>[2x]SMEDPDQLYTTLKNL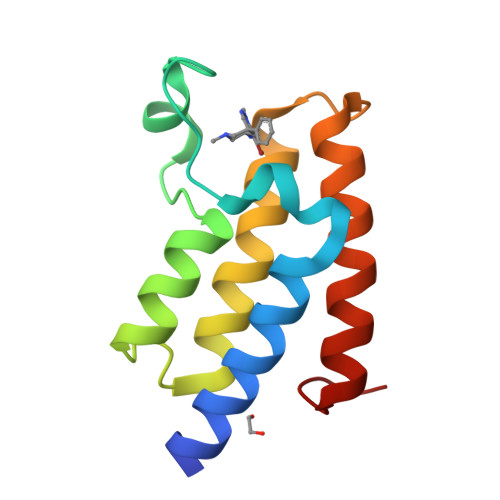LAQIKSHPSAWPFMEPVKKSEAPDYYEVIRFPIDLKTMTERLRSRYYVTRKLFVADLQRVIANCREYNPPDSEYCRCASALEKFFYFKLKEGGLIDK> MAHHHHHHEFPKPEFMSKSLEELQIGTYANIAMVRTTTPVYVALGIFVQHRVSALPVVDEKGRVV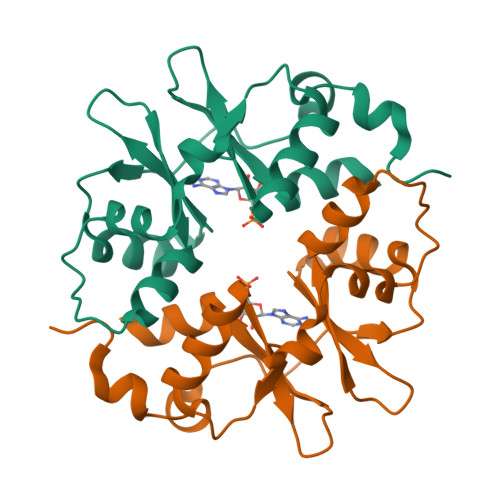DIYSKFDVINLAAEKTYNNLDVSVTKALQHRSHYFEGVLKCYLHETLETIINRLVEAEVHRLVVVDENDVVKGIVSLSDILQALVLT>GQDMVSPPPPIADEPLTVNTGIYLIECYSLDDKAETFKVNAFLSLSWKDRRLAFDPVRSGVRVKTYEPEAIWIPAIRFVNVENARDADVVDISVSPDGTVQYLERFSARVLSPLDFRRYPFDSQTLHIYLIVRSVDTRNIVLAVDLEKVGKNDDVFLTGWDIESFTAVVKPANFALEDRLESKLDYQLRISRQYFSYIPNIILPMLFILFISWTAFWSTS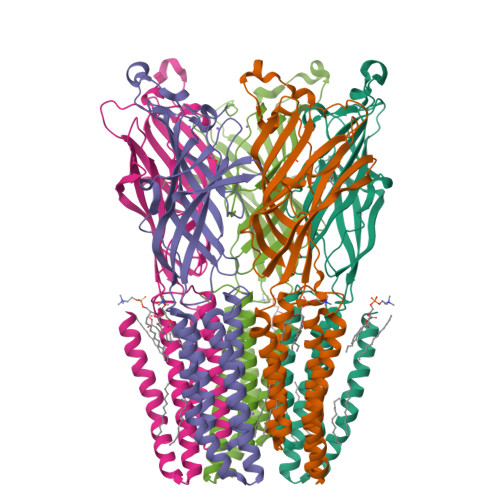YEANVTLVVSTLIAHIAFNILVETNLPKTPYMTYTGAIIFMIYLFYFVAVIEVTVQHYLKVESQPARAASITRASRIAFPVVFLLANIILAFLFFGF[5x]>[2x]MSFSSKPTVLASRVESDS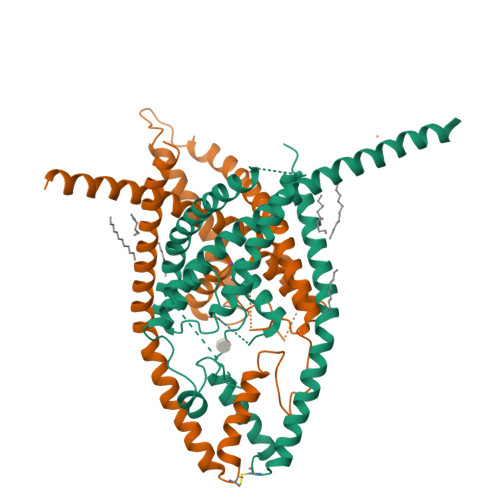AINVMKWKTVSTIFLVVVLYLIIGATVFKALEQPQEISQRTTIVIQREKFLRAHPCVSDQELDELIQQIVAAINAGIIPLGASSNQVSHWDLGSSFFFAGTVITTIGFGNISPRTEGGKIFCIIYALLGIPLFGFLLAGVGDQLGTIFGKGIAKVEDTFIKWNVSQTKIRIISTIIFILFGCVLFVALPAVIFKHIEGWSALDAIYFVVITLTTIGFGDYVAGGSDIEYLDFYKPVVWFWILVGLAYFAAVLSMIGDWLRVIAKKTKEAVGEFRAHAAEWTANVTSNSLEVLFQ> MSKLPQVKALYPYTAANDEELSFKVGDIITILEKDEGWWKGELNGQEG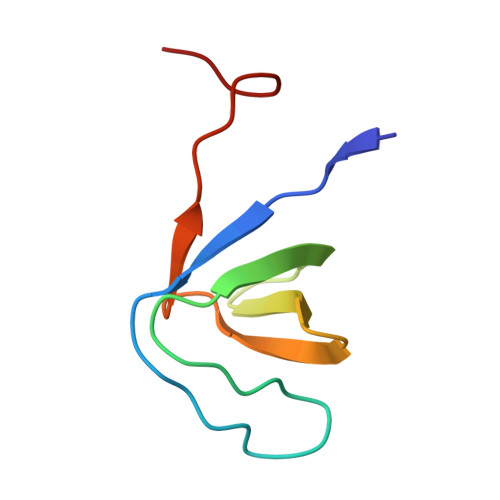WIPNNYVKEILEHHHHHH5'-O-{(S)-hydroxy[(prop-2-yn-1-yl)oxy]phosphoryl}adenosine 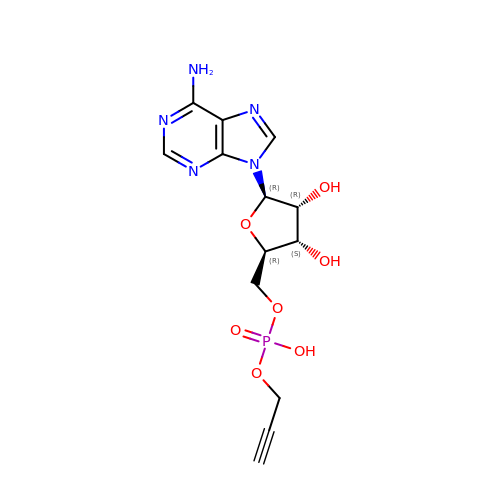| C13 H16 N5 O7 P | JGOCYNVVFDYFDU-QYVSTXNMSA-N Ribonucleotide reductases (RNRs) catalyze the conversion of ribonucleotides to deoxyribonucleotides, a conserved reaction that is fundamental to DNA-based life. Nearly all aerobic organisms use class I RNRs, which consist of two subunits: α, which contains the catalytic site, and β, which houses a subclass-dependent metal center. Contrary to all other class Ib RNRs studied to-date, the sole RNR of Bacillus subtilis displays class Ia-like activity regulation. We find that B. subtilis RNR has arrived at a remarkably similar solution to the ATP-cone through the evolution of two unique allosteric sites that modulate catalytic activity by inducing contrasting quaternary interactions that either enable or prevent the full range of motions needed for RNR activity.

In support of this, we screened 27 diffraction-quality crystals grown with various combinations of ATP, TTP, GDP, and CDP, and only those grown with GDP displayed electron density at the M-site. For example, no density was observed at this site in a 2.95 Å structure of the S-dimer obtained with CDP instead of GDP in the crystallization condition. However, the absence of nucleotide in the M-site of our 2.95 Å S-dimer structure suggests that ATP’s activating effect is primarily exerted by displacement of deoxyribonucleotides at the I-site. Conversely, the primary activating effect of ATP is to destabilize the I-dimer interface by displacing deoxyribonucleotides at the I-site. As ATP has a low affinity for the S-site, the combination of a specificity effector at the S-site and ATP at the I-site favors S-dimer formation.

>MSQNQVPKWIQLNNEIMIQKDGKFQFDKDKEAVHSYFVDYINQNTVFFHNLKEKLDYLVENQYYEEEFLSLYSFEDIKEVFKTAYAKKFRFPSFMSAFKFYNDYALKTNDKKKILERYEDRISIVALFFANGDTEKAKEYVNLMINQEYQPSTPTFLNAGRKRRGELVSCFLLEVNDSLNDISRAIDISMQLSKLGGGVSLNLSKLRAKGEAIKDVENATKGVVGVMKLLDNAFRYADQMGQRQGSGAAYLNIFHRDINDFLDTKKISADEDVRVKTLSIGVVIPDKFVELAREDKAAYVFYPHTIYKEYGQHMDEMDMNEMYDKFVDNPRVKKEKINPRKLLEKLAMLRSESGYPYIMFQDNVNKVHANNHISKVKFSNLCSEVLQASQVSSYTDYDEEDEIGLDISCNLGSLNILNVMEHKSIEKTVKLATDSLTHVSETTDIRNAPAVRRANKAMKSIGLGAMNLHGYLAQNGIAYESPEARDFANTFFMMVNFYSIQRSAEIAKEKGETFDQYEGSTYATGEYFDKYVSTDFSPKYEKIANLFEGMHIPTTEDWKKLKAFVAEHGMYHSYRLCIAPTGSISYVQSSTASVMPIMERIEERTYGNSKTYYPMPGLASNNWFFYKEAYDMDMFKVVDMIATIQQHIDQGISFTLFLKDTMTTRDLNRIDLYAHHRGIKTIYYARTKDTGQDSCLSCVV[2x]Here, we carried out a structural and functional characterization of the TOSV cap-snatching endonuclease, an N terminal domain of the viral polymerase (L protein) that provides capped 3′OH primers for transcription. We report TOSV endonuclease crystal structures in the apo form, in complex with a di-ketoacid inhibitor (DPBA) and in an intermediate state of inhibitor release, showing details on substrate binding and active site dynamics. The structure has significant rearrangements in the domain folding compared to previously reported EN structures. To better illustrate these changes, we show the structure in comparison with the EN domain of the homologous LACV, the prototype of the Orthobunyavirus genus, in Figure 2B and C. The TOSV EN fold is organised as two alpha-beta lobes rather than the one alpha/beta and one alpha bundle lobe architecture that is conserved in LACV EN and all previously described bunyaviral cap-snatching EN structures. The active site of the TOSV EN is defined by the H-D-PD-E-K motif, and maintains the canonical configuration observed in other His+ cap-snatching ENs.

SeMet derivatised DPBA co-crystals grew as thick plates that diffracted to 2 Å resolution and were thus used to solve the TOSV EN structure by single anomalous diffraction (SAD). The structure of the TOSV EN with DPBA shows the inhibitor binding through chelation of two Mn2+ in the active site of each molecule in the asu. The anomalous signal from the two metal ions is detected for both sites with similar intensities. The Mn2+ ion occupancies in the structure are of 1 and 0.72 for positions Mn1 and Mn2 respectively. Mn2 is octahedrally coordinated by the central D113 and two water molecules, in addition to D90 in the flexible loop, which swings into the active site and becomes ordered relative to the apo structure. When 0.5 mM of DPBA inhibitor was added, we detected a further increase in thermal stability of 10°C that was dependent on the presence of Mn2+ (Tm = 49.6 ± 0.2°C). Since DPBA forms no direct contacts to the protein, the increase in protein stability measured upon DPBA binding seems to be a result of the second manganese ion (Mn2) binding to the active site, induced by the inhibitor. Upon DPBA binding the number of bound sulphate ions is also reduced relative to the apo structure, thus suggesting a lower affinity for sulphate ions. Only SO4− is present in molB and no density is observed for SO42+ and SO43+ sulphate ions in molA and molB.

>GMERILKKQPAPVRALTIHPLRRYESSIYDTPIPAYVIKHSSDGVTIDIATSELADGQSGSTIQPFESVPAQNLTLFKHDFTFGHLADTTDKKFVEVFGVLENRADDSDFQSPDMIIETETGHVYVVEFTTTMGDANSADLAARNKIAKYEIACLDRSAIKPISLYIIAVHFNGVVSNLDLSDEEVNEIVFRFRLARDIFEELREINPALFD[2x]>MADIGSVLQKEGIEISEGTGYDLSKEPGAATVKALEQGTIVISYKTTSENAIQSLLSVGNGTKGNQDRHFHLYITNAGGVGMELRNTDGEFKYTLDCPAAVRGSYKGERVSNTVALKADKENKQYKLFANGELIATLDQEAFKFISDITGVDNVMLGGTMRQGTVAYPFGGSIERMQVYRDVLSDDELIAVTG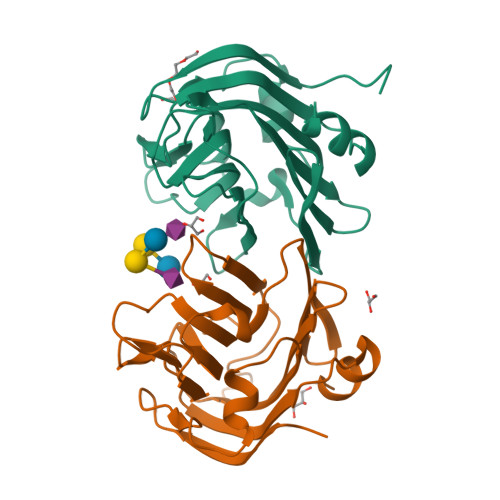K[2x]>[2x]GDKLDLSPIDYYGSGSYWKTEAQATAYIDGIHKHLRDAAWQHTITFGELRGGRFITGASSDGMGVSNGDIILQNFDETHTGVSKFGDLFGRITNLNLFIARVTDATYLSDEMKNFYLGEVYGLRAFYYFDLYRIYGGVPLRLTADVVEGVIDPNKLYMARSTPKEVMTQIKSDLNKSMEYFGNMNDFDPYKRGKKVYWSKAATECLMGEVYLWTSKVTTGDDVANPADLTIAKTHLESVLNNYNLKMLDDFSQVFNAKNKANDEIIFAIRFLEGEATNSNGTFTYNVGTGSTKNRYQANGEVFGDALDIQNTGNQTYEYNKAVYQNFDDADT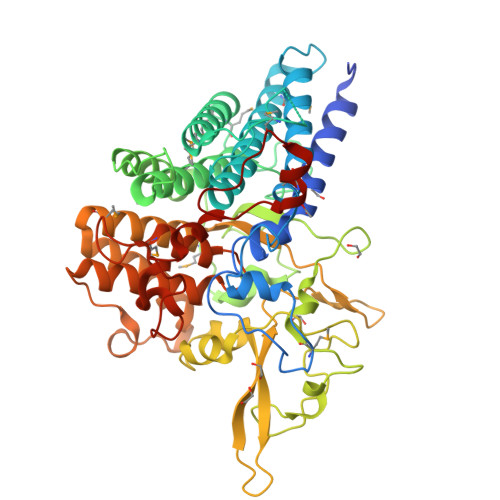RKEATFIASYNKDGKTGELSLYGTHVRKNIGYVNAQGARVYCGDYIFYRLPWVYLTLAEIANMEGDNAAVAKYINLVRKRAYGNAWDETLYAYPETADFTTNELAILHEKDKEFIQEGQRWWDLRRMTLTKGGTPLVFCKEGSLLGDAPILNKSTEAHKLLWPIEKTMLNKDPALEQTPGYK>[2x]MYLTLQEWNARQRRPR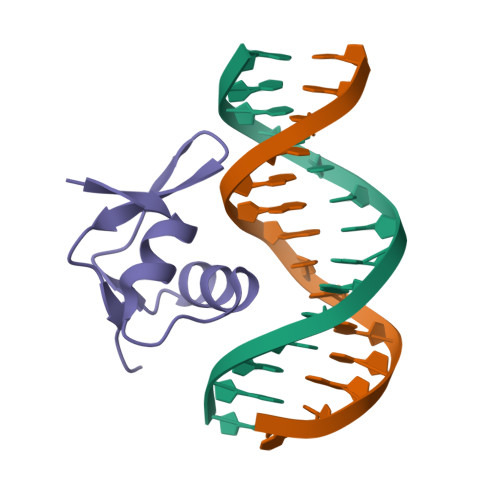SLETVRRWVRESRIFPPPVKDGREYLFHESAVKVDLNRP> APQQINDIVHRTITPLIEQQKIPGMAVAVIYQGKPYYFTWGYADIAKKQPVTQQTLFELGSVSKTFTGVLGGDAIARGEIKLSDPTTKYWPELTAKQWNGITLLHLATYTAGGLPLQVPDEVKSSSDLLRFYQNWQPAWAPGTQRLYANSSIGLFGALAVKPSGLSFEQAMQTRVFQPLKLNHTWINVPPAEEKNYAWGYREGKAVHVSPGALDAEAYGVKSTIEDMARWVQSNLKPLDINEKTLQQGIQLAQSRYWQTGDMYQGLGWEMLDWPVNPDSIINGSDNKIALAARPVKAITPPTPAVRAS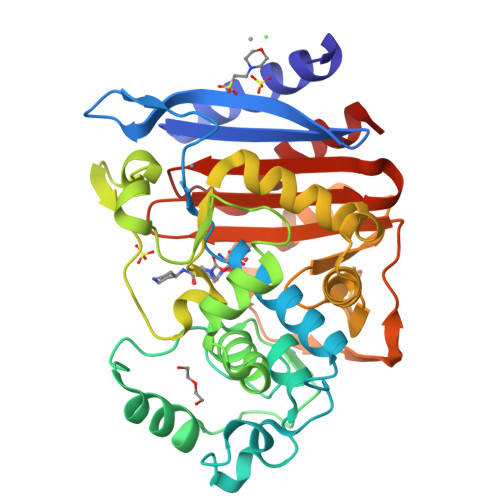WVHKTGATGGFGSYVAFIPEKELGIVMLANKNYPNPARVDAAWQILNALQ> MEYIIKNGFVYCPLNGVDGEKMDICVKDGKIVESVSDSAKVIDASGKIVMPGGVDPHSHIAGAKVNVGRMYRPEDSKRDAEKFKGGRAGSGFSVPSTFMTGYRYAQMGYTTAMEAAMPPLLARHTHEEFHDTPIIDHAAYPLFGNNWFVMEYLKEGDVDACAAYASWLLRATKGYTIKIVNPAGTEAWGWGGNVHGIYDPAPYFDITPAEIIKGLAEVNEKLQLPHSIHLHCNDLGHPGNYETTLASFDVPKNIKPNPATGSRDTVLYATHVQFHSYGGTTWRDFVSEAPKIADYVNKNDHIVIDVGQITLDETTTMTADGPMEYDLHSLNGLKWANCDVELETGSGVVPFIYSARAPVPAVQWAIGMELFLLIDNPEKVCLTTDSPNAGP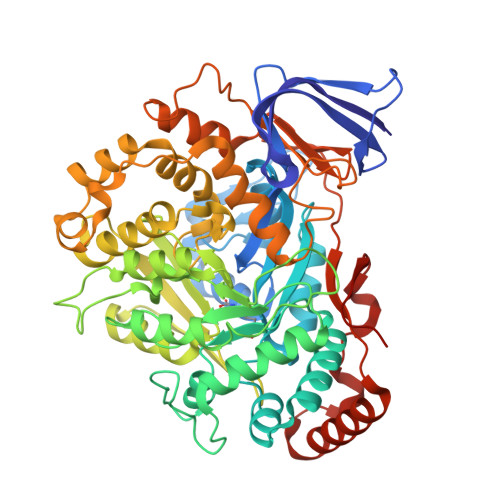FTRYPRVIAWLMSNKYRMNLIEGELHKWAQRKSTVATIDREYTFSEIAQITRATSAKVLGLSDTKGHLGVGADADIAVYDINPETVDPSAEYMAIEEAFSRAACVLKDGEIVVKDGEVVASPHGRTYWVDTQVDESIYSEVLANVESKFKQYYSVNFANYPVQDDYLPKSAPVKGVML>GSHMASLTEIEHLVQSVCKSYRETCQLRLEDLLRQRSNIFSREEVTGYQRKSMWEMWERCAHHLTEAIQYVVEFAKRLSGFMELCQNDQIVLLKAGAMEVVLVRMCRAYNADNRTVFFEGKYGGMELFRALGCSELISSIF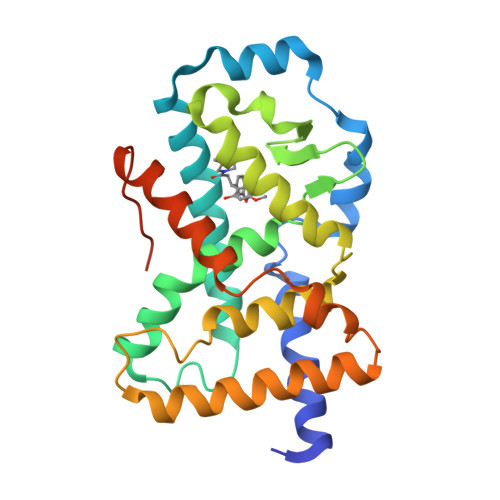DFSHSLSALHFSEDEIALYTALVLINAHRPGLQEKRKVEQLQYNLELAFHHHLCKTHRQSILAKLPPKGKLRSLCSQHVERLQIFQHLHPIVVQAAFPPLYKELFS[4x]>GSHMASRRFVLDTSVFTNPDVYLRFDEEPMQAISVFLGLARRADAEFYMPGPVYQELCNLR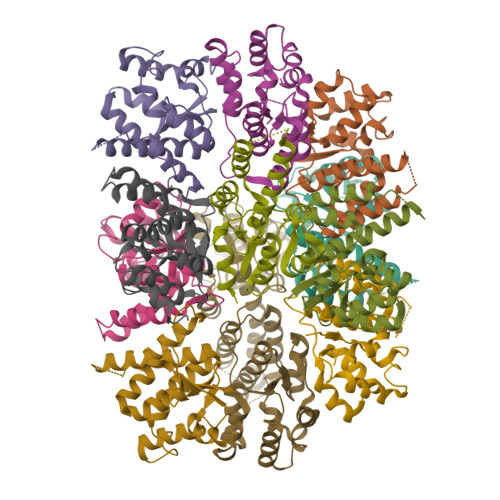SMDLIGAEFETEVYIRSPRRFSMTIPSEVLYEFIEEVRTRIQRGLRIAEEHARQAGQAESLPPELITQLRERYREAMRRGILDSREDIDVVLLAYELDATLVSADEGMRKFAERIGIKLVNPRYLRGVMQNLAGDDPGHAPPCGPDQPAG[12x]> MHHHHHHKNIINTSILNLRYESNHLIDLSRYASKINIGSKVNFDPIDKNQIQLFNLESSKIEVILKNAIVYNSMYENFSTSFWIRIPKYFNSISLNNEYTIINCMENNSGWKVSLNYGEIIWTLQDTQEIKQRVVFKYSQMINISDYINRWIFVTITNNRLNNSKIYINGRLIDQKPISNLGNIHASNNIMFKLDGCRDTHRYIWIKYFNLFDKELNEKEIKDLYDNQSNSGILKDFWGDYLQYDKPYYMLNLYDPNKYVDVNNVGIRGYMYLKGPRGSVMTTNIYLNSSLYRGTKFIIKKYASGNKDNIVRNNDRVYINVVVKNKEYRLATNASQAGVEKILSALEIPDVGNLSQVVVMKSKNDQGITNKCKMNLQDNNGNDIGFIGFHQFNN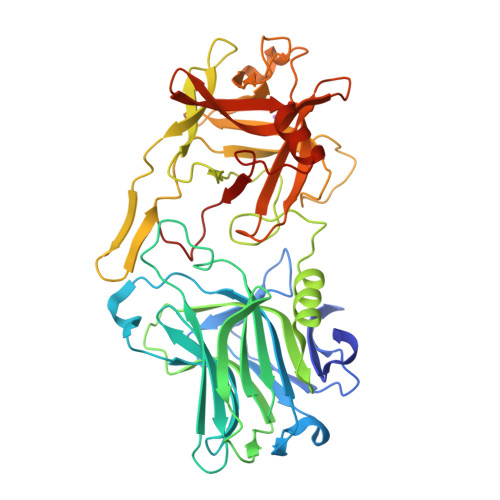IAKLVASNWYNRQIERSSRTLGCSWEFIPVDDGWGERPL> XIASASCTT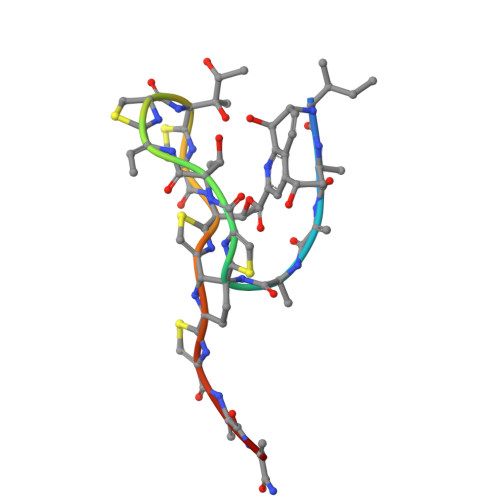CICTCSCSSX> MDIKNNLSDYTESEFLEIIEEFFKNKSGLKGS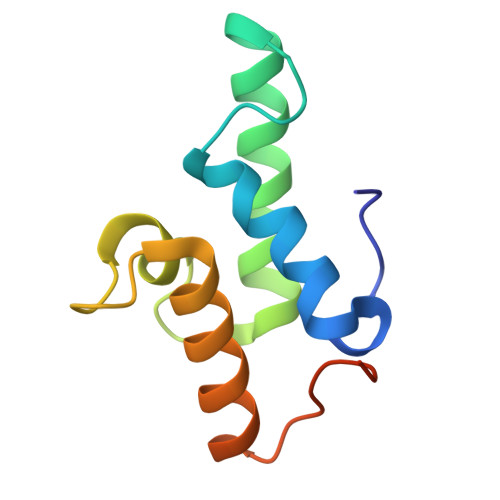ELEKRMDKLVKHFEEVTSHPRKSGVIFHPKPGFETPEGIVKEVKEWRAANGLPGFKAGLEHHHHHH Semaphorin-5A (Sema5A) is a bifunctional guidance cue exerting attractive and inhibitory effects on neuronal growth through the interaction with heparan sulfate (HS) and chondroitin sulfate (CS) glycosaminoglycans (GAGs), respectively. TSRs are a unique feature of Sema5s and enable interactions with heparan sulfate (HS) and chondroitin sulfate (CS) glycosaminoglycan (GAG) chains linked to the protein core of proteoglycans. We determined four Sema5ATSR3-4 crystal structures to high resolution (1.56–2.72 Å); apo state and complexes with nitrate, sulfate, and the heparin disaccharide mimetic sucrose octasulfate (SOS). Sema5ATSR3-4 is a rod-like dimer; superposition of the various structures indicates TSR3-TSR4 inter-domain angle differences, which may contribute conformational flexibility to the Sema5A ectodomain.

The novel architecture of TSR4 supports two symmetrically positioned ~20 × 20 Å-sized shallow cavities on the opposing sides of the Sema5A dimer. Positively charged and polar residues (K505, T732, K734, R747, R749) from both monomers contribute to each of these sites, together providing a notable positive electrostatic surface potential. Co-crystallization with SOS also resulted in this heparin surrogate occupying one of these sites in the Sema5ATSR3-4 dimer forming multiple electrostatic and polar interactions with the protein. Collectively, the three co-crystal structures indicate that these cavities constitute the focus for Sema5A GAG interactions.

>[2x]ETGPHMFWTGWGPWERCTAQCGGGIQARRRICENGPDCAGCNVEYQSCNTNPCPELKKTTPWTPWTPVNISDNGGHYEQRFRYTCKARLADPNLLEVGRQRIEMRYCSSDGTSGCSTGTLEVLFQ> MTEDLFGDLQDDTILAHLDNPAEDTSRFPALLAELNDLLRGELSRLGVDPAHSLEIVVAICKHLGGGQVYIPRGQALDSLIRDLRIWNDFNGRNVSELTTRYGVTFNTVY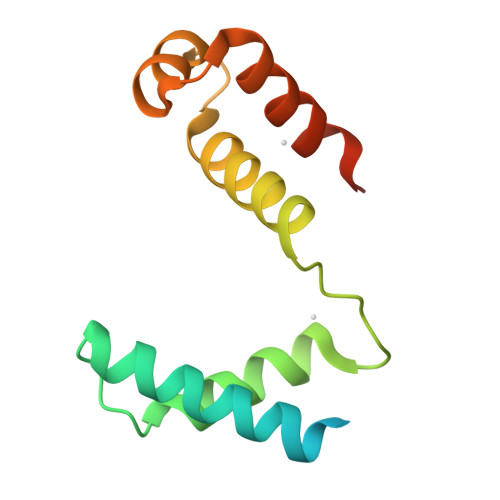KAIRRMRRLKYRQYQPSLL>[2x]QQLTYSQLVLRTAIQDQYSKLSGDGPFPMAFGLVLSEEERREVIDLYSLQFQYPDQPELQRLVILPQTHSTRTRRRAKGSYTWYLRSLNTNEMVCAVTIMAHHYETHHFVEVPL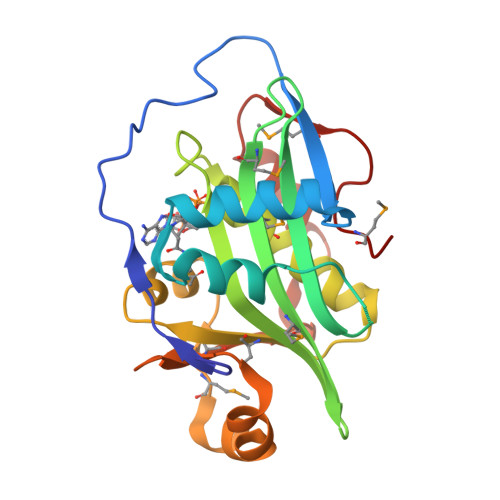FATGVGYKKHGFGRLMNAALLQWCVETGFEFVMISADVKAIPFWSHLGYKTMEKSELTRIVFYYEHNCYKFKGAEVMIRYCRTWPTDGVKEALARVQKVIVSGHVGLMDA>[4x]GPHMLDNFMKQ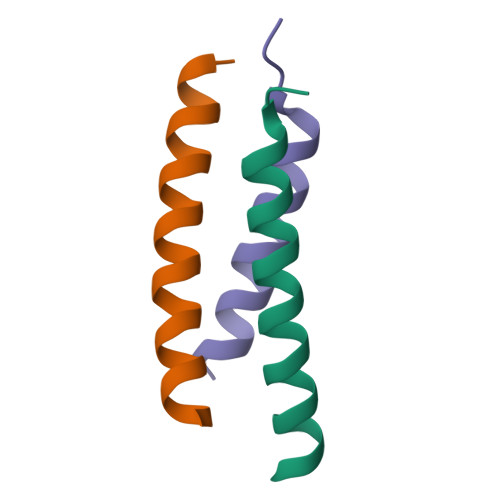LLKLEESLNKLELEQKVTNKE;>GPMEEQREILEQLKKTLQMLTVY[2x]> ATTLYENKTGTEDGYDYELWKDSGNTSMILNGGGTFSCQWSNINNCLFRKGKKFGGNQSYQQIGNISFDYGCDYHPNGNSYLCVYGWTTSPLVEFYIVDSWGSWRPPGGSPKGQIYVDGGTYDVYETTRVNQPSIQGNTTFQQYFSVRTERRTSGTINVTEHFKAWERMGMRMGNIYEAALNVEGYQSSGSANVYKNNMTIGGSSGQSGNQGGNQGGNQGGNQGGNTGSQTSGNETIVQCESMTKGGQYTGNINNPFGGVALYGNNDKVSYTQYFASGTHDFTLRGCSNNDNMARVDLKIGGETKGTFYYGGSYPAEYTIKNVNHGTGNQTIELVVTADNGQWDANIDYLKIGGAGVGGNESSGGNQGGNEGNQGGNAGNEGGNQAGNTGNQGGNEGNAGGQAQSGDNIVQCESMSKAGQYTGNINNPFDHHHHHH

We analysed a multidomain xylanase (Xyl) from the hindgut metagenome of the snouted harvester termite Trinervitermes trinervoides that releases xylobiose and xylotriose from beech and birch xylan and wheat arabinoxylan. The four domains of Xyl include an N-terminal GH11 xylanase domain, two family 36-like carbohydrate-binding domains CBM36-1 and 2, and a C-terminal CE4 esterase domain. Instead, individual domains and domain combinations were investigated structurally and for possible interdomain interactions. Xyl exemplifies a “beads-on-a-string” protein where the individual domains are “beads” each connected by a linker (string), with each domain retaining its individual function- making the synthesis of novel super enzymes for rapid and efficient degradation of bio-waste to biofuels within reach.

A two-domain construct, GH11-CBM36-1, previously cloned and biochemically characterised was structurally analysed in this study. Single crystals were obtained after three months using 10 mg/ml protein in 50 mM Na acetate pH 4.8, 0.5 M (NH4)2SO4 at 18°C. Diffraction data were collected on beamline ID29 at the European Synchrotron Radiation Facility (ESRF), Grenoble, France and automatically processed. The crystal structure of the GH11-CBM36-1 construct revealed electron density only for the GH11 domain and was refined to an R-free of 0.187 with a 99.9% completeness. This structure filled in the potentially missing information from the Xyl-GH11 domain above, which had a low completeness of 87.5%. Interestingly, the GH11 domains pack to create a hexagonal cylinder around the C-axis providing sufficient space for the CBM36-1 domains, however, the CBM36-1 could not be located. While the lack of electron density for the CBM36-1 domain could imply that the linker between the domains was degraded during crystallization, this is unlikely as GH11 would then presumably have crystallized in the same triclinic packing observed for the Xyl-GH11 domain above. The hexagonal packing of GH11-CBM36-1 has a solvent content of 69% and a Matthews coefficient of 4 (if GH11 only is considered), while the triclinic packing has a solvent content of 38% and a Matthews coefficient of 1.97. Thus, CBM36-1 potentially adopts a random orientation relative to the GH11 domain within the central void of the GH11 cylindrical tunnel. The 33-residue linker between GH11 and CBM36-1 is three times longer than the linker between the two domains in Xynj. The flexibility of the Xyl linker clearly prevents CBM36-1 being sandwiched in place within the crystal.[7,8-DIHYDRO-PTERIN-6-YL METHANYL]-PHOSPHONOPHOSPHATE | C7 H11 N5 O8 P2 | 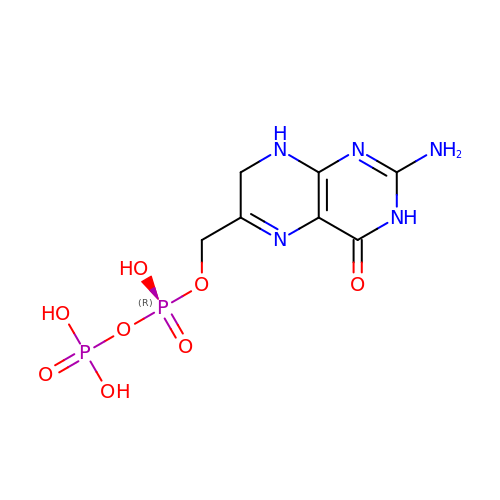FCQGJGLSOWZZON-UHFFFAOYSA-N> MDEIDLRILKILQYNAKYSLDEIAREIRIPKSTLSYRIKKLEKDGVIKGYYAYINPASLNLDYIVITSVKAKYGKNYHVELGNKLAQIPGVWGV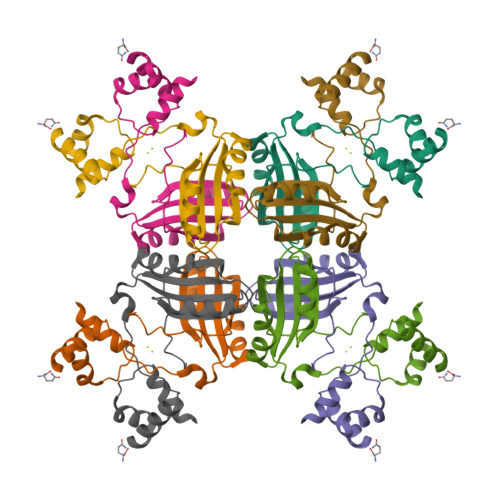YFVLGDNDFIVMARYKTREEFMEKFLERVMSIPEVERTSTQVVVKIIKESPNIVIF>[6x]MDCRNLCGAAAPSRLVQPGCFICRGVAVSIPPAAPGPATSVFDTPPSTFSLRPDGTIIAGTGIRGDHASVGTDGTIEMFIVPFIGDVTGSELTHPYAVELQDGEELAIAFGVTLKSGYGARITEYYDVSLFLENGGNSKELTLQPANTKSGYVWSDGHGYNITDSDGDLHTVQNVTRPVWFEMTEPGIVGVIMEARYKATGLVSSSISITVNVTYAD;>MNFNVGVDFPSFIAWDGEESFPVKVDGFNQFGFTFKTIAALTAATTFNIFYHEPSDADPCVPGPAIRVPEVPFCDTVLLSEDGLAAVTLPETVTPDSFCAGTVPCMNGQWISIAPATGSETNAANVQITVTMKGATR[30x];>[17x]MANKESELNGLDDIHSDIEKLSAH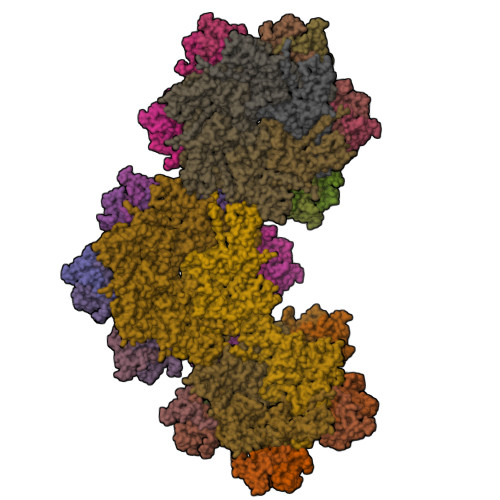VEKFSDGMDEKYKELTARFDGVKGDNDAIRKAVADATKEYAELSAKHQFFTEELAAMKARLDTPIMRSQAELDDHDRKTAIQLQRNMHEFRGGDPKEFVADESNLVDLKAYRSAVRKMLKVGIESKERVIASMTDVERKAFEASTIGPAFFTPQVLALEVDCNIECASLLDLYGQIEVSRSTFTYMKIADYGQLGEYTCDAKCDAEFGEPGNIRHLEGKTYDYRGVFCFNRKNLQEANYDFLSFMIGAAQRSHRINRNQALMIGKGVNEPKGWLTENCFPVFQTLPVDVNGTSTPAFLAQDWRRFVTSFPAEYGEARSVMHQNVFGYLAAMVDANGRFLFGDGDLTFTPDLVRERIRISNCLPDPTEGNTKGGTGQDAFAAGSFVAAQAAWKTAFYAVEKRPMFFEQYEGGSSAWCVKYQFGAEDGGFVGCCEHGRILQIG;>MVKLNCRPLCQAPTASRLVSPPCFICRGVAPSAPVTPG[11x]> SNAMKNYYSSNPTFYLGIDCIIFGFNEGEISLLLLKRNFEPAMGEWSLMGGFVQKDESVDDAAKRVLAELTGLENVYMEQVGAFGAIDRDPGERVVSIAYYALININEYDRELVQKHNAYWVNINELPALIFDHPEMVDKAREMMKQKASVEPIGFNLLPKLFTLSQLQSLYEAIYGEPMDKRNFRKRVAEMDFIEKTDKIDKLGSKR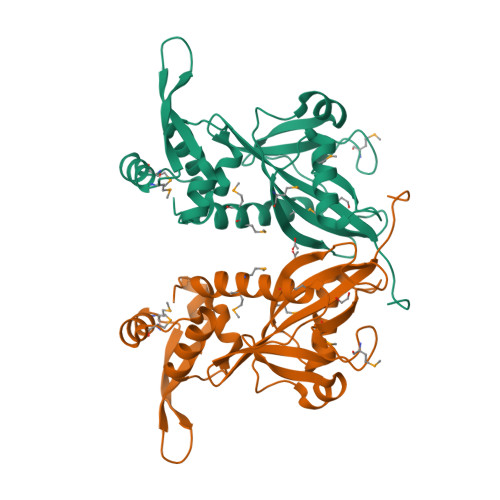GAALYKFNGKAYRKDPKFKL>GGGGCCGGGGCC[2x]

The abnormal GGGGCC hexanucleotide repeat expansions (HREs) in C9orf72 cause the fatal neurodegenerative diseases including amyotrophic lateral sclerosis and frontotemporal dementia. The transcribed RNA HREs, short for r(G4C2)n, can form toxic RNA foci which sequestrate RNA binding proteins and impair RNA processing, ultimately leading to neurodegeneration. Here, we reported the crystal structure of an eight-layer parallel tetrameric RNA G-quadruplex formed by two repeats of C9orf72 HRE RNA, r(G4C2)2, in K+ solution. Therefore, obtaining high-resolution structural information about the r(G4C2)n G-quadruplex is crucial for understanding the pathogenesis of ALS/FTD and developing more effective therapeutic approaches.

Finally, we successfully solved the crystal structure of r(G4C2)2 in the space group of P6122 with the resolution of 2.96 Å. There are two chains of r(G4C2)2 oligonucleotides in the asymmetric unit of the crystal. Intriguingly, chains A/B and their crystallographically symmetric molecules (chains A’/B’) form a parallel-stranded dimeric G-quadruplex unit (i.e. chains A/A’, chains B/B’), which is composed of four G-tetrads connected by two CC double-chain-reversal loops. The dimeric G-quadruplex unit co-axially stacks on the other crystallographically symmetric dimeric G-quadruplex unit in a 5′-to-5′ arrangement, resulting in a tetrameric eight-layer G-quadruplex through π–π interactions. The G1 base in one dimeric block stacks (i.e. chains A/B) with the G7 base in the opposite dimeric block (i.e. chains A’/B’). Interestingly, the base stacking mode at the interface is ‘Partial 5-ring’ in the crystal structure of r(G4C2)2, which is the first experimentally observed. Notably, the electron density was well defined for the nine equal-spaced K+ ions lying along the axis within the central core of the tetrameric G-quadruplex including well-defined central channel potassium ions located in the interface between the two dimeric blocks. Seven K+ ions locate in the G-core of the tetramer coordinating to eight neighbouring guanine O6 atoms at a distance of ∼2.8 Å leading to an anti-prismatic coordination environment. Interestingly, another two K+ ions coordinate to four neighbouring guanine O6 atoms of the outer G-tetrad at a distance of ∼3.2 Å and bridge the two cytosine in the 3′-end. For the two cytosine bases located at 3′ end of each stand, only C11 base was well defined in the electron density and stacks on G-tetrad of the dimeric block.>GSHHKAVLAVRREDVNAWERRAPLAPKHIKGITNLGYKVLIQPSNRRAIHDKDYVKAGGILQEDISEACLILGVKRPPEEKLMSRKTYAFFSHTIKAQEANMGLLDEILKQEIRLIDYEKMVDHRGVRVVAFGQWAGVAGMINILHGMGLRLLALGHHTPFMHIGMAHNYRNSSQAVQAVRDAGYEISLGLMPKSIGPLTFVFTGTGNVSKGAQAIFNELPCEYVEPHELKEVSQTGDLRKVYGTVLSRHHHLVRKTDAVYDPAEYDKHPERYISRFNTDIAPYTTCLINGIYWEQNTPRLLTRQDAQSLLAPGKFSPAGVEGCPALPHKLVAICDISADTGGSIEFMTECTTIEHPFCMYDADQHIIHDSVEGSGILMCSIDNLPAQLPIEATECFGDMLYPYVEEMILSDATQPLESQNFSPVVRDAVITSN[2x]

AASS is a bifunctional enzyme with an N-terminal lysine-2-oxoglutarate reductase (LOR) domain and a C-terminal saccharopine dehydrogenase (SDH) domain, which are homologous to Saccharomyces cerevisiae LYS1 and LYS9, respectively. The LOR domain catalyses the reductive deamination of L-lysine and 2-oxoglutarate into saccharopine (EC 1.5.1.8), which constitutes the first committed, and possibly rate-limiting, step in lysine degradation. The LOR domain itself consists of two lobes, both Rossman folds with a central beta-sheet with alpha helices on the outside. Moreover, AASS is a unique drug target for inborn errors of metabolism such as glutaric aciduria type 1 that arise from deficiencies downstream in the lysine degradation pathway.

We initially purified a short construct (amino acids 21–451) that expressed well in E. coli with high purity and a monodisperse peak on gel filtration. Importantly, we solved the first crystal structure of the human LOR domain at 2.2 Å resolution. The overall structure of the human protein is quite similar to yeast LYS1 despite the low sequence identity, indicating strong conservation of function despite the evolved differences such as adopting bifunctional enzyme architecture and switching from NAD+ to NADP+. Some of the extended loops and predicted catalytic residues were not visible in this structure. Moreover, when we tested this short construct for activity, we discovered that, despite the fact that it was well folded and aligned nicely with the yeast structure, it had no activity in our in vitro assay. (a) Asymmetric unit of the short inactive construct shows a dimer of the LOR domain of AASS. We reanalysed the structure of the short construct and noticed that although the interface in the asymmetric unit is likely non-physiologic, the interface of a monomer with its crystallographic symmetry-mate is identical to the long interface in the tetramer, further supporting the validity of this interface. One paradox to resolve was why the C-terminus is so critical for activity, despite the fact that it is distant from the active site and the shorter construct is well folded.>MSTTGTTPATTGYAAEFAGRTALVTGAASGIGLATARRLGAGGARVVVADFNAEGAEKAAAELRAGGVEAAAVELDVTRPESVEAAVGFAVDTFGSLDLAVNNAGIGGPSAPTGEYDVAAYQRVVRTNLDGVFYSMRYELPAIEAAGKGGSIVNVASILGSVGFAGSPAYVAAKHGVVGLTKAAAAEYAARGIRINAVGPGFIDTPLLKTMEEAAYKGLVALHPAGRLGRSDEVAELIVFLLSDRASFVAGSYHLVDG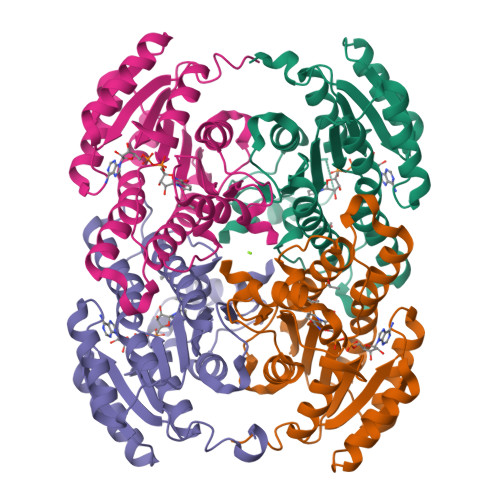AYTAV[12x]>AKPDRSSFVPSLFSKKKKNVTMRSIKTTRDRVPTYQYNMNFEKLGKCIIINNKNFDKVTGMGVRNGTDKDAEALFKCFRSLGFDVIVYNDCSCAKMQDLLKKASEEDHTNAACFACILLSHGEE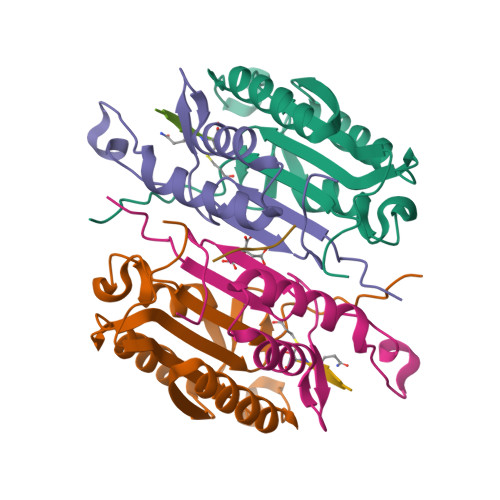NVIYGKDGVTPIKDLTAHFRGDRCKTLLEKPKLFFIQACRGTELDDGIQ[2x];>ANPRYKIPVEADFLFAYSTVPGYYSWRSPGRGSWFVQALCSILEEHGKDLEIMQILTRVNDRVARHFESQSDDPHFHEKKQIPCVVSMLTKELYFSQ[2x];> QGHGE>[8x]MSLKPVIGITGNRLVKGVDVFYGHRVTYTQQRYVDAIQKVGGFPIALPIDDPSTAVQAISLVDGLLLTGGQDITPQLYLEEPSQEIGAYFPPRDSYEIALVRAALDAGKPIFAICRGMQLVNVALGGTLYQDISQVETKALQHLQRVDEQLGSHTIDIEPTSELAKHHPNKKLVNSLHH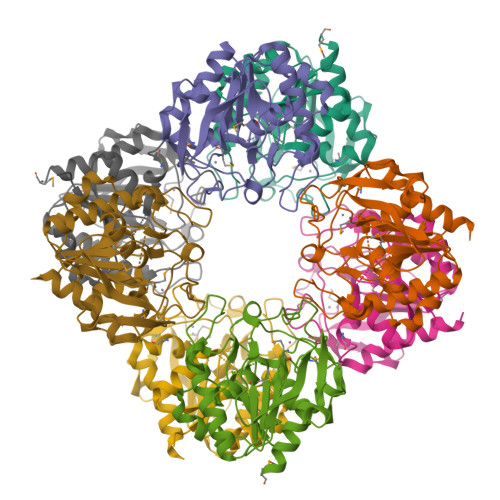QFIKKLAPSFKVTARTADGMIEAVEGDNLPSWYLGVQWHPELMFQTDPESEQLFQALVDESKKTMVKEGHHHHHH> MHHHHHHSSGRENLYFQGHMYKPVSLFLFFLILAAAIHTNAVQSADEAISKAAVLIRQPWLNEVMTGITHLGASSFLLPLIVIIGAGMFFYRKTWDGLLMLLVFGTDRLLNKVLKEWIERVRPDFAPLVHESSFSFPSGHSMNAACVYPVIAYFLVKHLPFLSKHKKMVYIIAGVIAVLVGISRVYLGVHFVTDVLGGFSLGLLLFFLVKGFDEKIKRFRQK

Responding to this critical need, we introduce here a fully automated method for collecting, selecting, and merging data from hundreds to thousands of in meso-grown microcrystals. This approach boosts the collective phasing signal of many tiny crystals to a level where de novo phasing of highly challenging membrane protein targets becomes not only possible but also fast and high-throughput. We refer to it as the in meso in situ serial crystallography—experimental phasing (IMISX-EP) method. IMISX-EP has three components: (1) in meso crystallization (and in situ soaking where appropriate), (2) fast, automated grid scanning, and serial data collection in situ, and (3) real-time data processing and selection of data sets followed by structure solution.

IMISX-EP using heavy atom co-crystallization was demonstrated with BacA and PgpB. PgpB was pre-incubated with Na2WO4 and subsequently crystallized in the cubic mesophase. The crystal used for data collection was relatively large and measured 10 × 50 × 150 μm3. As the crystal had its flat face oriented approximately parallel to the windows of the well, it was possible to record 140° of data using a rotation angle of ± 70° from this one crystal without compromising data quality at high-tilt angles. Because of the strong anomalous signal from tungsten and the high diffraction resolution, the structure was solved with the relatively low redundancy of 2.6 and a completeness of 91% with SHELXD/E. This example shows that the IMISX-EP approach can be used with large single crystals. The strength of the phasing signal, as estimated by the Bijvoet ratio, ranges from 1% in the case of native-SAD PepTSt to 7% for tungsten phasing of PgpB. Therefore, experimental phasing becomes considerably more difficult in going from working with the high-resolution data available for heavy atom-labeled W-PgpB to the mid-resolution data available for native S-PepTSt.> TTIVALTYKGGVLLAGDRRATQGNLIASRDVEKVYVTDEYSAAGIAGTAGIAIELVRLFAVELEHYEKIEGVPLTFDGKANRLASMVRGNLGAAMQGLAVVPLLVGYDLDADDESRAGRIVSYDVVGGRYEERAGYHAVGSGSLFAKSALKKIYSPDSDEETALRAAIESLYDAADDDSATGGPDLTRGIYPTAVTITQAGAVHVSEETTSELARRIVAERTEQG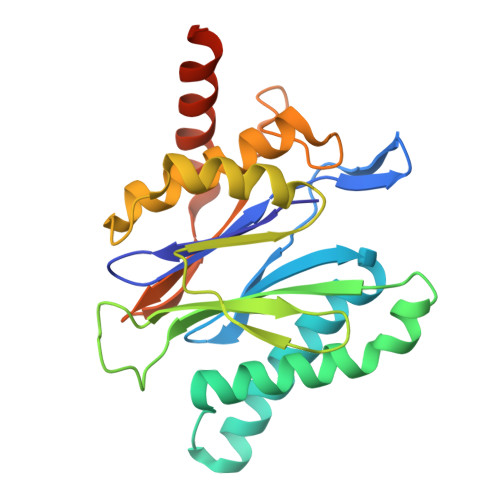GSARHHHHHH> GSHMGKRVLIVDDAAFMRMMLKDIITKAGYEVAGEATNG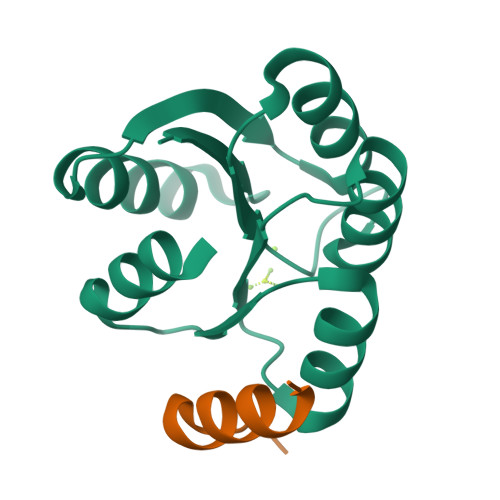REAVEKYKELKPDIVTMDITMPEMNGIDAIKEIMKIDPNAKIIVCSAMGQQAMVIEAIKAGAKDFIVKPFQPSRVVEALNKVSK;> MSDVLSQEEINQLIEALMKG>DSDLYAELRCLCIKTTSGIHPKNIQSLEVIGKGTHCNQVEVIATLKDGRKICLDPD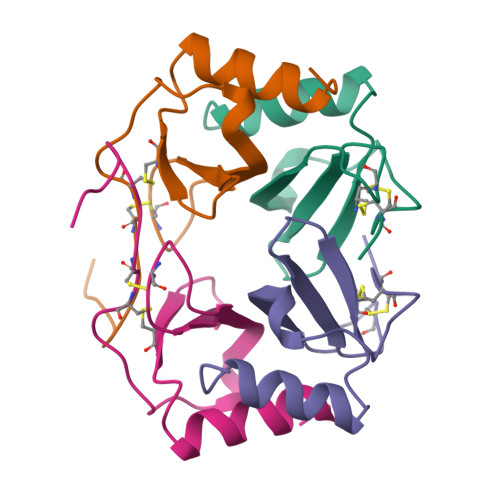APRIKKIVQKKLAGDESAD[4x]>[3x]AAVINTFDGVADYLQTYHKLPDNYITKSEAQALGWVASKGNLADVAPGKSIGGDIFSNREGKLPGKSGRTWREADINYTSGFRNSDRILYSSDW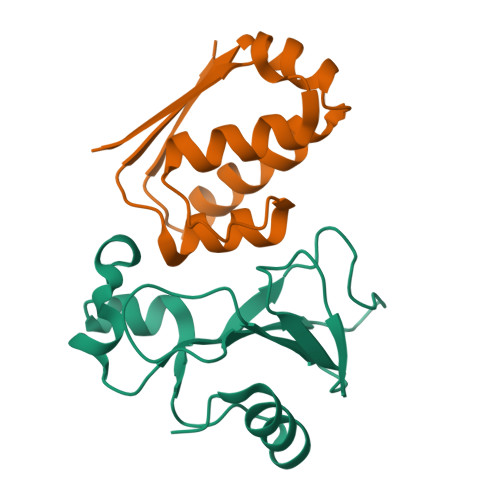LIYKTTDHYQTFTKIR;>[3x]MKKAVINGEQIRSISDLHQTLKKELALPEYYGENLAALWDALTGWVEYPLVLEWRQFEQSKQLTENGAESVLQVFREAKAEGADITIILS> GSGIALSRLAQERKAWRKDHPFGFVAVPTKNPDGTMNLMNWECAIPGAAGTPWAGGLFKLRMLFKDDYPSSPPKCKFEPPLFHPNVYPS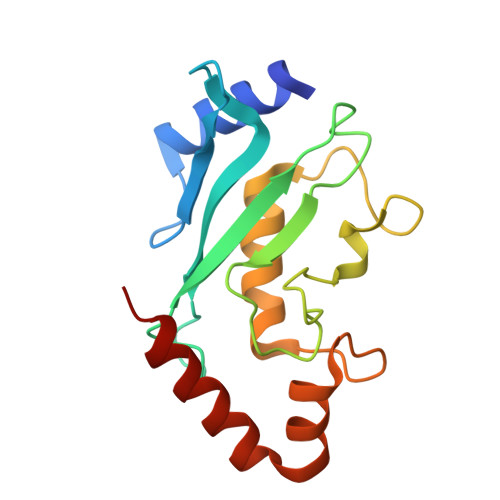GTVCLSILEEDKDWRPAITIKQILLGIQELLNEPNIQDPAQAEAYTIYAQNRVEYEKRVRAQAKKFAPS> MARVTVQDAVEKIGNRFDLVLVAARRARQMQVGGKDPLVPEENDKTTVIALREIEEG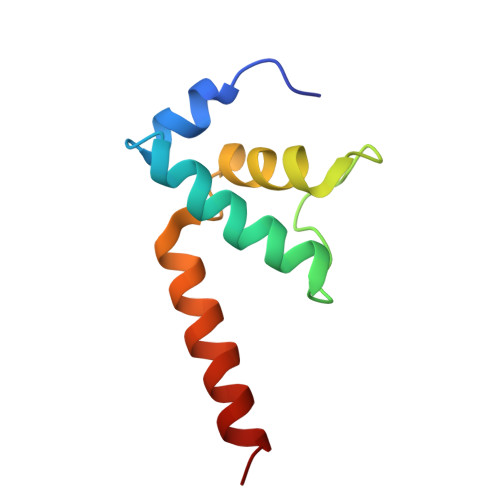LINNQILDVRERQEQQEQEAAEL>MLGLGGAATRQLTFQTSSPAHLTMPYVMPGDGEVVGVGEPVAIRFDENIADRGAAEKAIKITTNPPVEGAFYWLNNREVRWRPEHFWKPGTAVDVAVNTYGVDLGEGMFGEDNVQTHFTIGDEVI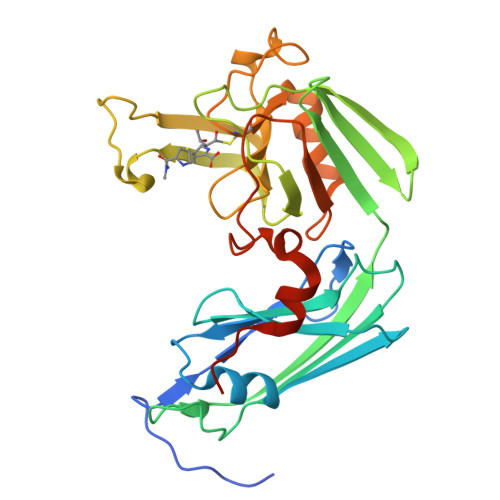ATADDNTKILTVRVNGEVVKSMPTSMGKDSTPTANGIYIVGSRYKHIIMDSSTYGVPVNSPNGYRTDVDWATQISYSGVFVHSAPWSVGAQGHTNTSHGCLNVSPSNAQWFYDHVKRGDIVEVVNTVGGTLPGIDGLGDWNIPWDQWRAGNAKALEHHHHHH[2x]methyl [(4S)-4-(3'-ethyl-6-fluoro[1,1'-biphenyl]-2-yl)-4-hydroxy-4-{(3R)-1-[4-(methylamino)butanoyl]piperidin-3-yl}butyl]carbamate 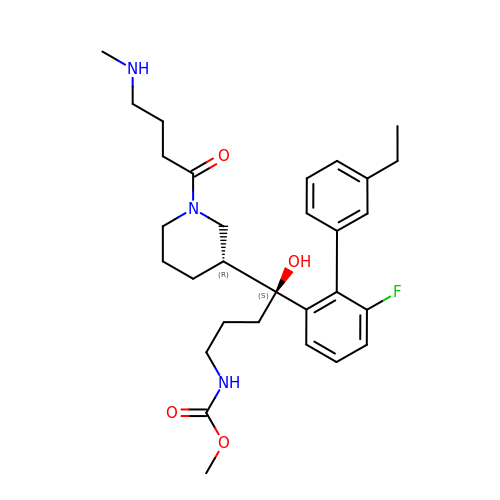| C30 H42 F N3 O4 | ZTHQDSYJEPZECE-HLADLETHSA-N> MAWPKVQPEVNIGVVGHVDFGKTTLVQAITGIWTSKHSEELKRGMTIKLGYAETNIGVCESCKKPEAYVTEPSCKSCGSDDEPKFLRRISFIDAPGHEVLMATMLSGAALMDGAILVVAANEPFPQPQTREHFVALGIIGVKNLIIVQNKVAVVSKEEALSQYRQIKQFTKGTWAENVPIIPVSALHKINIDSLIEGIEEYIKTPYRDLSQKPVMLVIRSFDVNKPGTQFNELKGGVIGGSIIQGLFKVDQEIKVLPGLRVEKQGKVSYEPIFTKISSIRFGDEEFKEAKPGGLVAIGTYLDPSLTKADNLLGSIITLADAEVPVLW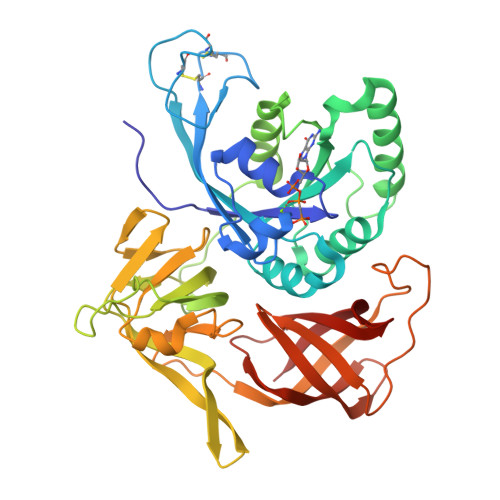NIRIKYNLLERVVGAKEMLKVDPIRAKETLMLSVGSSTTLGIVTSVKKDEIEVELRRPVAVWSNNIRTVISRQIAGRWRMIGWGLVEI>GEEQMRLPSADVYRFAEPDSEENIIFEENMQPKAGIPIIKAGTVIKLIERLTYHMYADPNFVRTFLTTYRSFCKPQELLSLIIERFEIPEPEPTEADRIAIENGDQPLSAELKRFRKEYIQPVQLRVLNVCRHWVEHHFYDFERDAYLLQRMEEFIGTVRGKAMKKWVESITKIIQRKKIARDNGPGHNITFQSSPPTVEWHISRPGHIETFDLLTLHPIEIARQLTLLESDLYRAVQPSELVGSVWTKEDKEINSPNLLKMIRHTTNLTLWFEKCIVETENLEERVAVVSRIIEILQVFQELNNFNGVLEVVSAMNSSPVYRLDHTFEQIPSRQKKILEEAHELSEDHYKKYLAKLRSINPPCVPFFGIYLTNILKTEEGNPEVLKRHGKELINFSKRRKVAEITGEIQQYQNQPYCLRVESDIKRFFENLNPMGNSMEKEFTDYLFNKSLEIEPRNPKPLPRFPKKYSYPLKSPGVRPSNPRPGT[2x]

SOS1 is one of the major guanine nucleotide exchange factors that regulates the ability of KRAS to cycle through its “on” and “off” states. One of the major regulators of this process is the Son of Sevenless (SOS) protein, a guanine nucleotide exchange factor (GEF) that acts as a key activator for KRAS function. The binding between KRAS and SOS proteins helps facilitate the turnover of GDP-loaded KRAS into its GTP-loaded state. Additionally, functional genomic screens have identified that several cancer cell lines addicted to KRAS signaling are particularly sensitive to genetic perturbation of SOS1.15 Functionally, KRAS mutations lead to a reduction in GTPase activity, resulting in a higher population of GTP-bound KRAS and increased RAS-pathway signaling. GTP-bound KRAS also binds to an allosteric site on SOS1, leading to an increase in SOS1 GEF activity, thereby ensuring a high population of active KRAS. Herein, we report the design of a new class of phthalazine-based SOS1 binders that effectively disrupt the SOS1:KRAS protein–protein interaction.

Pushing out from the 3-position of the phenyl ring with a bromo substituent was well tolerated for SOS1 binding, and further introduction of the 3-cyano substituent resulted in the highly potent inhibitor of the SOS1:KRAS PPI, MRTX0902 (32), with a reduced lipophilicity (cLogP = 3.4). Based on the pKa of MRTX0902 (measured pKa = 6.7, ∼17% ionized at pH 7.4), the phthalazine is not highly protonated under physiological conditions; however, the local acidic environment of the protein likely helps drive protonation of the phthalazine core. The structure further revealed that the newly installed 3-cyano substituent on the phenyl ring presumably enhances the edge-to-face interaction with Phe890 due to the electron-withdrawing nature of the 3-cyano substituent. The substituted phenyl ring also provides shape complementary with the back pocket of SOS1, although the cyano substituent creates no discernible interactions with the protein as captured in the static structure. The SAR of the benzyl amine modifications show that the 3-cyano substituent in 32 provided the most effective combination of potency and lipophilicity and led to a nearly 6-fold decrease in CYP3A4 inhibition (IC50 = 3.6 μM) when compared to that of the 3-trifluoromethyl-substituted phenyl 24. Furthermore, the co-crystal structure of MRTX0902 (32) suggested that the C6-position on the phthalazine could be used to further tune the electronics of the core structure. Further in vitro profiling showed that MRTX0902 (32) was highly selective for SOS1 when compared to SOS2 and showed no inhibition of EGFR. X-ray co-crystal structures of these inhibitors reveal a unique salt bridge between the phthalazine core and Glu902 of SOS1 that has not been reported with previous SOS1 binders.>[12x]KLTLWTTPDPSPNCQLLSDRDAKFTLCLTKCGSQILGTVAVAAVTVGSALNPINDTVKSAIVFLRFDSDGVLM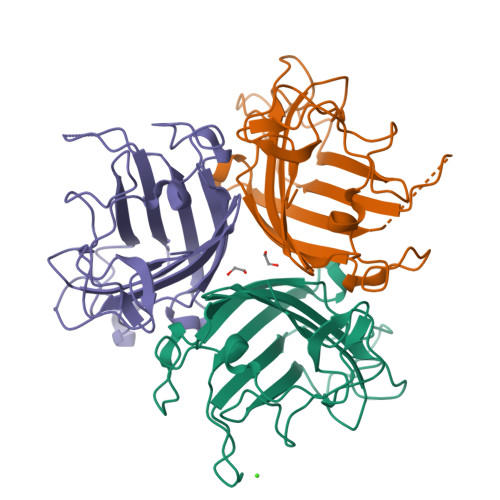SNSSMVGDYWNFREGQTTQSVAYTNAVGFMPNLGAYPKTQSKTPKNSIVSQVYLNGETTMPMTLTITFNGTDEKDTTPVSTYSMTFTWQWTGDYKDKNITFATNSFTFSYMAQE>MGHHHHHHHHHHSSGHIEGRHMMATNLRGVMAALLTPFDQQQALDKASLRRLVQFNIQQGIDGLYVGGSTGEAFVQSLSEREQVLEIVAEEAKGKIKLIAHVGCVSTAESQQLAASAKRYGFDAVSAVTPFYYPFSFEEHCDHYRAIIDSADGLPMVVYNIPALSGVKLTLDQINTLVTLPGVGALKQT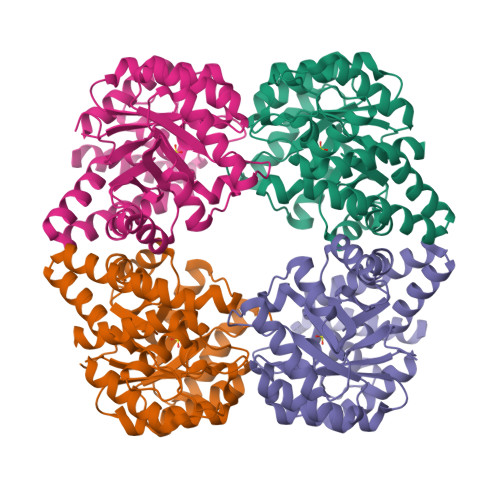SGDLYQMEQIRREHPDLVLYNGYDEIFASGLLAGADGGIGSTYNIMGWRYQGIVKALKEGDIQTAQKLQTECNKVIDLLIKTGRFRGLKTVLHYMDVVSVPLCRKPFGPVDEKYLPELKALAQQLMQERG[4x]>GAMAMITPSERSVETNGVRLRLVEAGERGDPLVVLAHGFPELAYSWRHQIPALVDAGYHVMAPDQRGYGGSSAPEAIEAYDITRLTADLMGLLDDIGAEKAAFIGHDWGALVVWNAALLYPDRVAAVAGLSVPPVPRSLTRPTEAFRALVGEDNFFYILYFQEPGVADAELDGDPARTMRRMFGGLTSDPDAAHRMLQPGPAGFIDRLPEPEALPDWLTAEELDHYIAEFTRTGFTGGLNWYRNMDRNWELTEHLAGATITAPALFLAGAADPVLGFMRPERATEVAVGPYRQVLLDGAGHW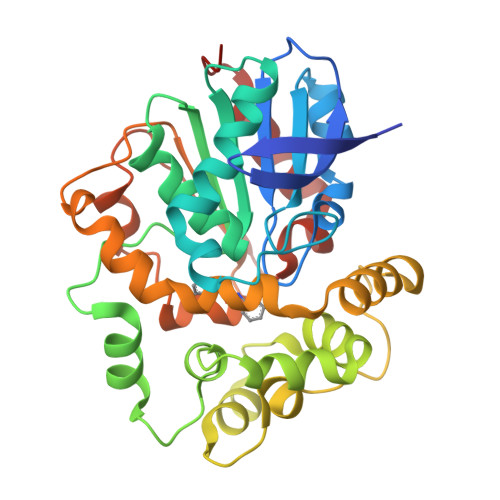VQQERPQEVNAALIDFLRGLELQ[4x]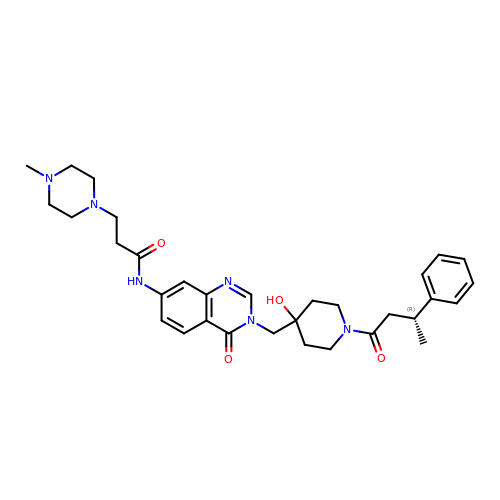N-[3-({4-hydroxy-1-[(3R)-3-phenylbutanoyl]piperidin-4-yl}methyl)-4-oxo-3,4-dihydroquinazolin-7-yl]-3-(4-methylpiperazin-1-yl)propanamide | C32 H42 N6 O4 | QLBYDWATOPNXBG-XMMPIXPASA-N> MDKEAFLERVREGAELIKMHIELGHTIRLISHRDADGITAGAILAKAVAREGGTFQLSIVKQVSEELIDQLAREKREIYVFSDLGSGSIELIEEKLNFATVVVADHHPPEKDSFSTDSHVLVNPVPFGANSVRDLSGSGVAYFVAREMNRKNRDMAYVAIVGAVGDMQEIDGTFHGLNLEIIEDGKELGILEVRKELRLFGRESRPLYQMLAYATNPEIPEITGDERKAIEWLRAKGFDPEMKYWQLREEEKRKLHEALLVHMIKHGAPKEAIDRLIGDVVISPLYPEGDVRHEAREFATLLNATGRLNAGTLGVAICLGDEEAYKVARKMLDDYKKEQIEARKFIIQNWNMVEEGEHAYVFYAGKNIRDTLVGIAANMAINAGLADPEKPVVVLADSDEDENLVKG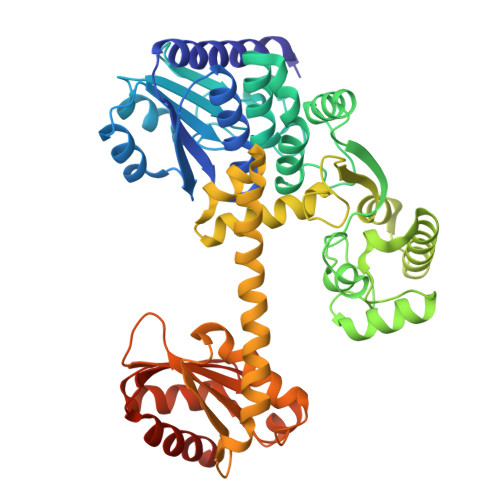SARTTEKALEKGYHLGEALKEVAEKLGGEGGGHAIAAGIRFPKNRIDEFIKLFNEALGRQVKGGGSEGEG FtfL is a key enzyme in C1 metabolism pathway. It catalyzes the synthesis of formyltetrahydrofolic acid from formic acid and tetrahydrofolic acid. Formyltetrahydrofolic acid is then converted through two reactions to 5,10-methylene tetrahydrofolic acid, a metabolite for biosynthesis of pyrimidines and amino acids. PaFtfL exhibits a tetramer in all three crystal structures, consistent with other reported FtfL crystal structures.

We subsequently determined the crystal structure of PaFtfL complexed with BBR and found that BBR binds at both the “allosteric site” and “active site” of PaFtfL and thereby likely inhibits PaFtfL via interfering conformational flexibility of PaFtfL tetramer and competing with its substrate ATP. In the crystal structure of PaFtfL-BBR, the Fo-Fc electron density difference map clearly shows three types of binding sites of BBR. In the first type of binding site, named as “active site,” two molecules of BBR occupy the active site of protomers B and D, respectively, in which BBR mainly makes Van der Waals interactions with surrounding residues (T74, N381, F383, P384, W411). Specifically, the B ring of BBR is sandwiched between the aromatic side chains of residues F383 and W411. Structural comparison among our crystal structures of PaFtfL-BBR, PaFtfL-ATP, and MtFtfL-folate suggests that BBR overlaps with ATP and tetrahydrofolate on binding to FtfL, indicating that BBR likely competes with ATP and tetrahydrofolate to bind FtfL active site. The biochemical assay also showed that the apparent Michaelis constants (Km) of ATP and tetrahydrofolate increased when BBR was added, supporting that BBR inhibits the enzymatic activity of FtfL partially through direct competition. Each BBR molecule also makes Van der Waals interactions with the side-chain atoms of surrounding residues (N153, P159, V189). The presence of BBR in the protomer interface causes a 4.4° rotation of one dimer towards the other. We infer that the binding of BBR at the subunit interface might contribute to its inhibition on PaFtfL catalytic reaction through allosteric effect, and simultaneous binding at both allosteric and active sites explains the potent inhibition of BBR on PaFtfL. In addition, in the third type of binding site, named as “crystal-packing site,” two molecules of BBR locates between two crystal symmetry-related tetramers of FtfL, and thereby we infer that the interaction is not relevant to its inhibitory function.

>[2x]GSHMMEFKTDIEIAQEANPQDIRDIAKKINLSEDDIELYGKYKAKIDYNVLNRTKSRAGKLILTTAINPTPAGEGKTTTSIGVADALAKLGKNVIAALREPSMGPVFGIKGGAAGGGYAQVVPMEDINLHFTGDMHAIGAANNLLAAMLDNHVYQTNSLNINPKRITWRRCVDMNDRQLRNVVDGLGKKVDGVTREDGFDITVASEVMAAFCLSNNISELKENLGNIVVAYNYSGKPVTARDLNAHGAMAAILKDALKPNLVQTLEGTPAILHGGPFANIAHGCNSIIATKMGMHMADYVVTEAGFGADLGAEKFLDIKCRKAGIRPDAVIIVATVRALKYNGGVAKDQLNNENLEALEKGLPNLLKHIENITQVYKIPAVVAINRFPLDTDAELALVRSKCEELGVKVALSEVWANGGEGGIEVANEVLKLIEEGENNFEYCYEEDMTIKEKLNAIATKIYGADGVNYTKEANKQIAELEELGFGNLPVCVAKTQYSLSDDQTKLGRPTGFTIEVRQANISAGAGFVVVMTGEIMKMPGLPKLPAAERIDVDENGKISGLF>TFQERLLAFERKHVITPEAHVTLAKQLAGDIALELQAYLRSKFPELPFGALVPGGPLYDGLQAGTAEHVRLLAPLELEPGLWSLVPGVDTVAAEPRCWAVRRTQLEFHPRGCSPWDRFLVGGYLSSRVLLELLRKALSASVNWPAIGSLLGCLIWPDVASEELLLKVQHECLEFTLAVLMVVPGASTDDRLLLAWPLEGLASNLWLQDLYPVETARLRALDDQD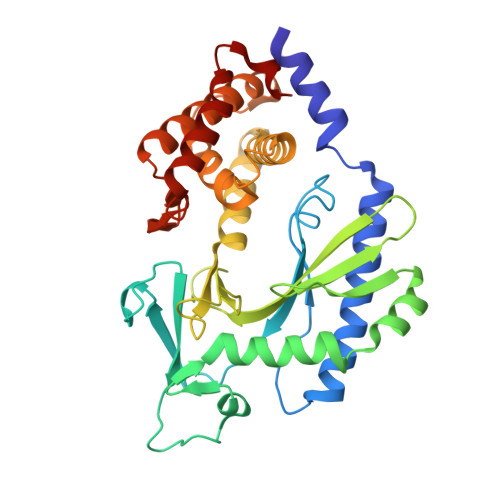AGTRRRLLLLLCGICRGHPALVRLGWSHLTQVVLHLGEEEVAWTEEALGERFLQALEFLVGSLEQASLPCHFNPSVNLLGNFREEEIDDIGYVLYSGLQVPESLF[2x]>[2x]MHHHHHHHHHHGTDDDDKMAATVAVDNLNPKVLKCEYAVRGEIVIHAQRLQEQLKTQPGSLPFDEILYCNIGNPQSLGQQPVTFFREVLALCDHPDLLQREEIKTLFSADSISRAKQILAMIPGRATGAYSHSQGIHGLRDAIAS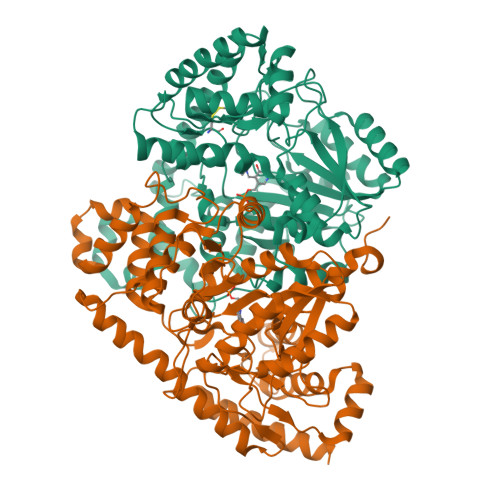GIASRDGFPANADDIFLTDGASPGVHLMMQLLIRNEKDGILVPIPQYPLYSASIALHGGALVPYYLNESTGWGLETSDVKKQLEDARSRGINVRALVVINPGNPTGQVLAEENQYDIVKFCKNEGLVLLADEVYQENIYVDNKKFHSFKKIVRSLGYGEEDLPLVSYQSVSKGYYGECGKRGGYFEITGFSAPVREQIYKIASVNLCSNITGQILASLVMNPPKASDESYASYKAEKDGILASLARRAKALEHAFNKLEGITCNEAEGAMYVFPQICLPQKAIEAAKAANKAPDAFYALRLLESTGIVVVPGSGFGQVPGTWHFRCTILPQEDKIPAVISRFTVFHEAFMSEYRD> MTAAAFDDLRPRLGRLTEETIDIAREVLVE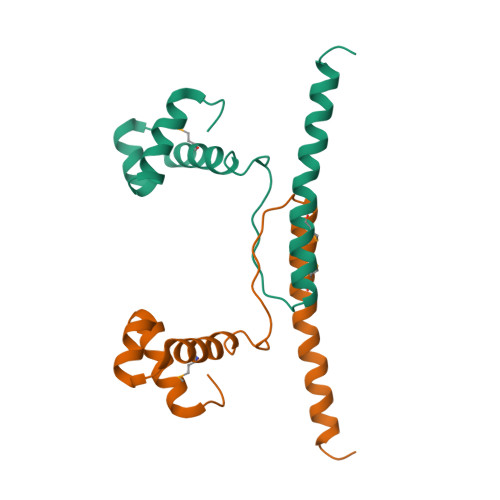GKSQSDVARERGLSRQRVSSMVKSVVSAANEIPREWQRVEVWLPPNLAEKVRQMEADAKADVARKNQLTDAALEHHHHHH> MGSSHHHHHHSSGLVMDPETVRIAL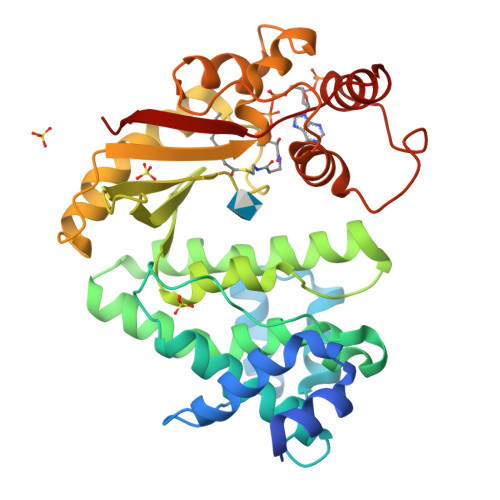GLEERTAAWLTELDELGPPAEPVRLPRGEEARDLLRRLEVPELDAEEIVAAAPDPDRDPALWWLLERTHHAIVRHMGDHRAKPRGGPPLPYEGGAAARYFHVYVFLATVPAVRRFHAERGIPDEVGWETLTQLGELVAIHRRKYGQGGMNMQWWTTYHLRGILYRLGRLQFSLATGKDGTPHLGLHVPEWGGPLLPKAYDESLHRARPFFDRHFPEHGARVAWGSSWMLDPQLEEYLTEDSNIIQLARFWTLTDSAPEPGNADGDSSILEFVFRYNGQPLDELPQRSSLERAVIAHLKAGRHWHMRTGFVKLP> SGPRGPRKCARKTRHAETS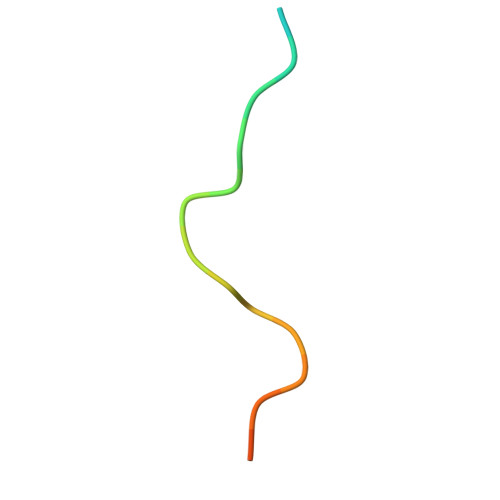GA N-[2-(cyclohexyloxy)-4-nitrophenyl]methanesulfonamide 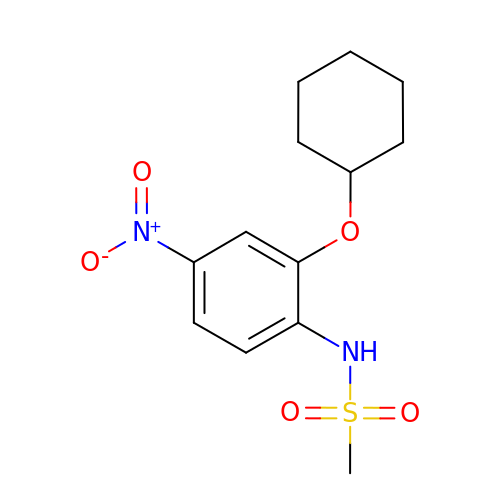| C13 H18 N2 O5 S | KTDZCOWXCWUPEO-UHFFFAOYSA-N> MSVQQIDWDLALIQKYNYSGPRYTSYPTALEFSEDFGEQAFLQAVARYPERPLSLYVHIPFCHKLCYFCGCNKIVTRQQHKADQYLDALEQEIVHRAPLFAGRHVSQLHWGGGTPTYLNKAQISRLMKLLRENFQFNADAEISIEVDPREIELDVLDHLRAEGFNRLSMGVQDFNKEVQRLVNREQDEEFIFALLNHAREIGFTSTNIDLIYGLPKQTPESFAFTLKRVAELNPDRLSVFNYAHLPTIFAAQRKIKDADLPSPQQKLDILQETIAFLTQSGYQFI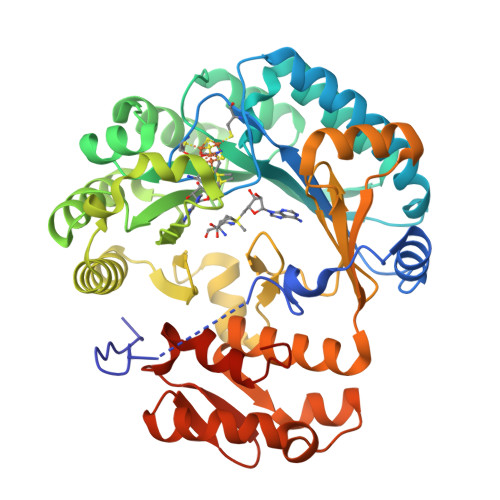GMDHFARPDDELAVAQREGVLHRNFQGYTTQGDTDLLGMGVSAISMIGDCYAQNQKELKQYYQQVDEQGNALWRGIALTRDDCIRRDVIKSLICNFRLDYSPIEQQWDLLFADYFAEDLKLLAPLAKDGLVDVDEKGIQVTAKGRLLIRNICMCFDTYLRQKARMQQFSRVI> GQYDDHPPVFQKKFYIGGVSEDARMFASVLRVKATDRDTGNYSAMAYRLIIPPIKEGKEGFVVETYTGLIKTAMLFHNMRRSYFKFQVIATDDYGKGLSGKADVLVSVVNQLDMQVIVSNVPPTLVEKKIEDLTEILDRYVQEQIPGAKVVVESIGARRHGDAYSLEDYSKCDLTVYAIDPQT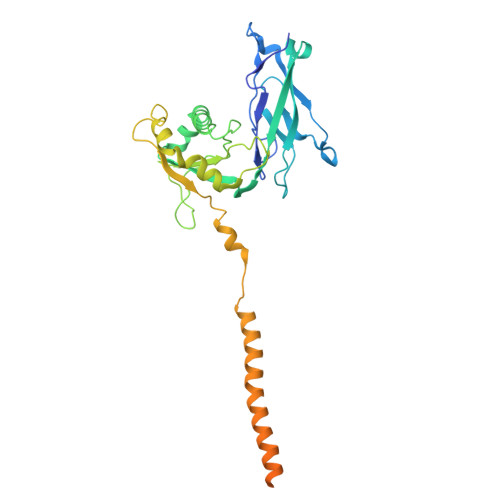NRAIDRNELFKFLDGKLLDINKDFQPYYGEGGRILEIRTPEAVTSIKKRGESLGYTEGALLALAFIIILCCIPAILVVLVSYRQFKVRQAECTKTARIQSAMPAAKPAAPVPAAPAPPPPPPPPPPGAHLYEELGESAMHKYETALFESRLVPR> MGSSHHHHHHSQDPHMAMEMRLPVARKPLSERLGRDTKKHLVVPGDTITTDTGFMRGHGTYMGEEKLIASVAGSVERVNKLICVKALKTRYIGEVGDIVVGRITEVQQKRWKVETNSRLDSVLLLSSMNLPGGELRRRSAEDELAMRGFLQEGDLISAEVQAVFSDGAVSLHTRSLKYGKLGQGVLVQVSPSLVKRQKT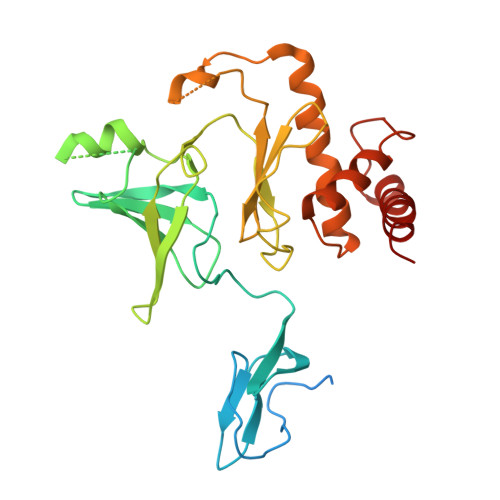HFHDLPCGASVILGNNGFIWIYPTPEHKEEEAGGFIANLEPVSLADREVISRLRNCIISLVTQRMMLYDTSILYCYEASLPHQIKDILKPEIMEEIVMETRQRLLEQEG>[5x]MVEELKRKLRQAKEDGDEELLERVKNEMLLLAVVDPRVLVEVLNTAKELGDEEMYKKVKGIMLRLAVVDPRVLVLVLELAEALGDEEMKEKVKNIMLLLAVVDPRVLVLVLELAEELGDEEMKKEVEEILDKLAEVDPRVAVLKEVAKKEGSWLEHHHHHH

Here we describe a systematic approach to generating modular and rigid repeat protein oligomers with coincident C2 to C8 and superhelical symmetry axes that can be readily extended by repeat propagation. Repeat proteins are composed of an asymmetric structural motif that is concatenated several times in tandem within a single protein chain. From these building blocks, we demonstrate that a wide range of unbounded fibres can be systematically designed by introducing hydrophilic surface patches that force staggering of the monomers; the geometry of such fibres can be precisely tuned by varying the number of repeat units in the monomer and the placement of the hydrophilic patches. All multiplexes follow the naming convention CsHRN_Rr where s is the cyclic symmetry, HR stands for helical repeat, R is the number of repeats in a single chain and N is an index to differentiate between multiplexes of the same symmetry.

We determined the high-resolution structures of five designs from C2 to C6 symmetry by X-ray crystallography, cryogenic electron microscopy (cryoEM) or both. The C5HR2_4r interface is focused near the inner radius of the structure, and is composed of a thin strip of hydrophobic residues along the helical axis; desolvated salt bridges also line the inner radius of C5HR2_4r. C5HR2_4r has the largest helical rise parameter of the structures, with an average helical rise of 1.1 nm per repeat. C5HR2_4r matches the design model with an overall C-alpha r.m.s.d. of 2.11 Å and has a Vr of 12.6, higher than that of the other designs, further suggesting that all 12 designs are close to the correct structure.>GSKKLAEYKCNTNTAIELKLVRFPEDLENDIRTFFPEYTHQLFGDDETAFGYKGLKILLYYIAGSLSTMFRVEYASKVDENFDCVEADDVEGKIRQIIPPGFCTNTNDFLSLLEKEVDFKPFGTLLHTYSVLSPTGGENFTFQIYKADMTCRGFREYHERLQTFLMWFIETASFIDVDDERWHYFLVFEKYNKDGATLFATVGYMTVYNYYVYPDKTRPRVSQMLILTPFQGQGHGAQLLETVHRYYTEFPTVLDITAEDPSKS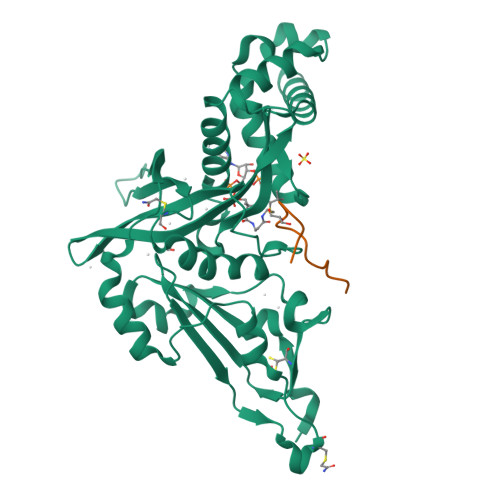YVKLRDFVLVKLCQDLPCFSREKLMQGFNEDMAIEAQQKFKINKQHARRVYEILRLLVTD[2x];>SGRGKGGKGLGAGGAKRHRK[2x]> SDQTWVQCDACLKWRKLPDGMDQLPEKWYCSNNPDPQFRNCEVPEEPED;> ARTKQ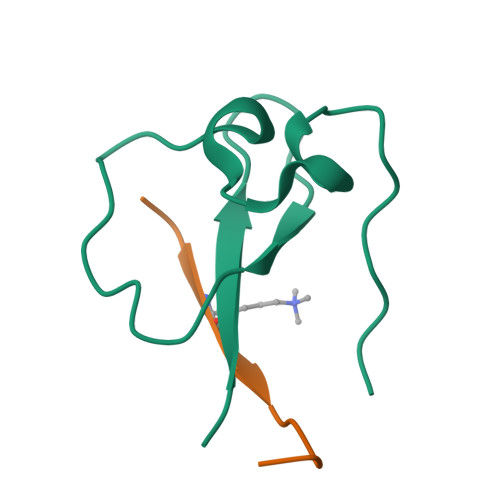TARKST>AKVATGTDILSAASNVSLQKARTWDEGVESKFSTTPVNDIFKDKKVVIFGLPGAYTGVCSSKHVPPYKHNIDKFKAKGVDSVICVAINDPYTVNAWAEKIQAKDAIEFYGDFDGS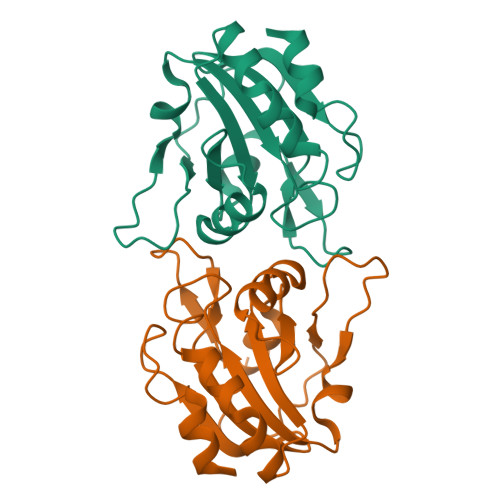FHKSLELTTDLSAGLLGIRSERWSAYVVDGKVKALNVEESPSDVKVSGAETILGQI[6x]> MEIVYKPLDIRNEEQFASIKKLIDADLSEPYSIYVYRYFLNQWPELTYIAVDNKSGTPNIPIGCIVCKMDPH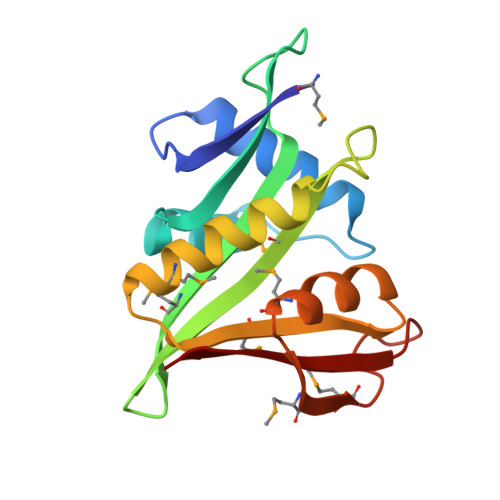RNVRLRGYIGMLAVESTYRGHGIAKKLVEIAIDKMQREHCDEIMLETEVENSAALNLYEGMGFIRMKRMFRYYLNEGDAFKLILPLT> MAKLTALTLLGMGLALFDRQKSSFQTRFNVHREVTPVELPNCNLVKGIDNGSEDLEILPNGLAFISSGLKYPGIMSFDPDKSGKILLMDLNEKEPAVSELEIIGNTLDISSFNPHGISTFIDDDNTVYLLVVNHPGSSSTVEVFKFQEEEKSLLHLKTIRHKLL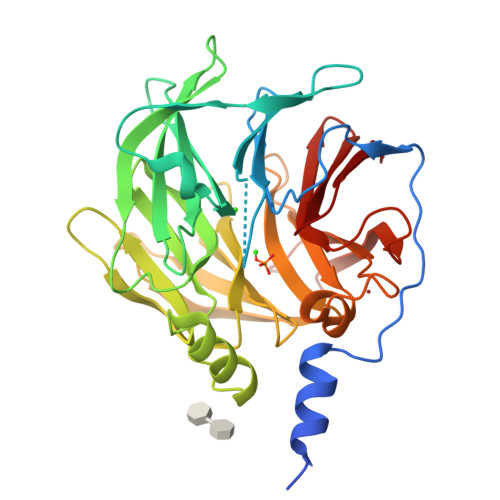PSVNDIVAVGPEHFYATNDHYFIDPYLKSWEMHLGLAWSFVTYYSPNDVRVVAEGFDFANGINISPDGKYVYIAELLAHKIHVYEKHANWTLTPLRVLSFDTLVDNISVDPVTGDLWVGCHPNGMRIFFYDAENPPGSEVLRIQDILSEEPKVTVVYAENGTVLQGSTVAAVYKGKLLIGTVFHKALYCDL> MALFSCFRCGYMYEFAVSNSYCRKLTL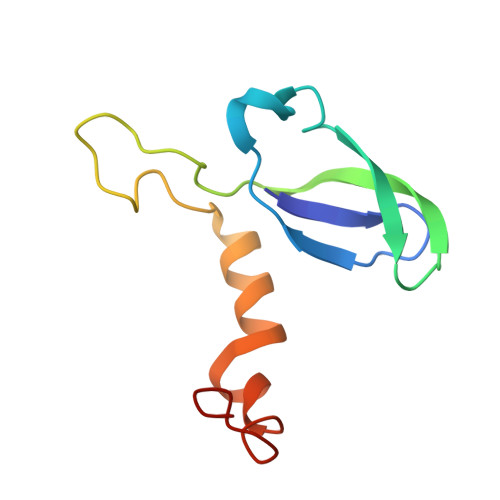RNDHCPRCDQLTLFRFMSVSGMVGNMPFKPIGVPGPSYATLWWRKTREGKEASAPLDAVCKSDRW> GPLGSEAHLYMQVQIVAEDQFCGHQGNDMYDEEKVKYTVFKVLKNSSLAEFVQSLSQTMGFPQDQIRLWPMQARSNGTKRPAMLDNEADGNKTMIELSDNENPWTIFLETVDPELAASGATLPKFDKDHDVMLFLKMYDPKTRSLNYCGHIYTPISCKIRDLLPVMCDRAGFIQDTSLILYEE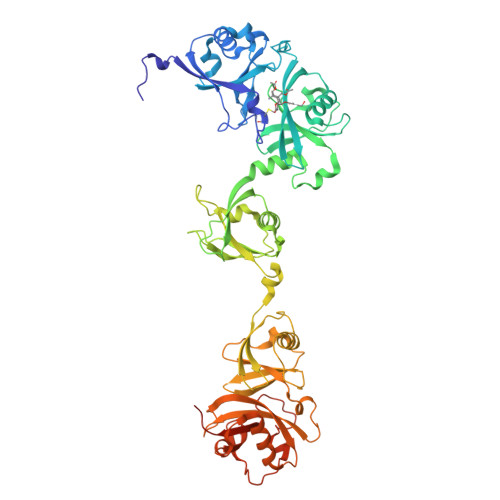VKPNLTERIQDYDVSLDKALDELMDGDIIVFQKDDPENDNSELPTAKEYFRDLYHRVDVIFCDKTIPNDPGFVVTLSNRMNYFQVAKTVAQRLNTDPMLLQFFKSQGYRDGPGNPLRHNYEGTLRDLLQFFKPRQPKKLYYQQLKMKITDFENRRSFKCIWLNSQFREEEITLYPDKHGCVRDLLEECKKAVELGEKASGKLRLLEIVSYKIIGVHQEDELLECLSPATSRTFRIEEIPLDQVDIDKENEMLVTVAHFHKEVFGTFGIPFLLRIHQGEHFREVMKRIQSLLDIQEKEFEKFKFAIVMMGRHQYINEDEYEVNLKDFEPQPGNMSHPRPWLGLDHFNKAPKRSRYTYLEKAIKIHN> MRRNILLVQFVGVLLLLPSIMSGQQHSSDNKNWAEKGIVIREVEILGKRPMKDIGVQQTRFDSLVLKENIALSMADILTFNSSIFVKSYGRATLSTVSFRGTSASHTQVTWNGMRINNPMLGMTDFSMIPSYFIDDASLLHGTSSVNMAGGGLGGLVKLSTVPAHQEGFGMQYVQGIGSFSTFDEFLQLKYGDKHWQISTRAVYQSSPNDYKYRNHDKKENIYDDKYNIIEQYYPIERNRSGAYKDLHILQEVYYNTGKGDRFGLNAWYTDSNRELALLTTDQGDLMDFENRQREHTLRSVLSWDHTRENWKVSARGGYVHTWLAYDYKRDLGNGIMATMTRSRSKVNTFYGQLDGEYFFSDKLLLTAGVSAHQHLVNSLDKDLNKDDNKNDKYGQGRKNDSIVYFDKGRIELSGNVSLKWQPVNRLGMSLVLRGEMFGTKWAPVIPAFFVDYVLSKRGNIMAKASITRNYRFPTLNDLYFLPGGNPALNNESGFTYETGLSFSVDKDNVYTL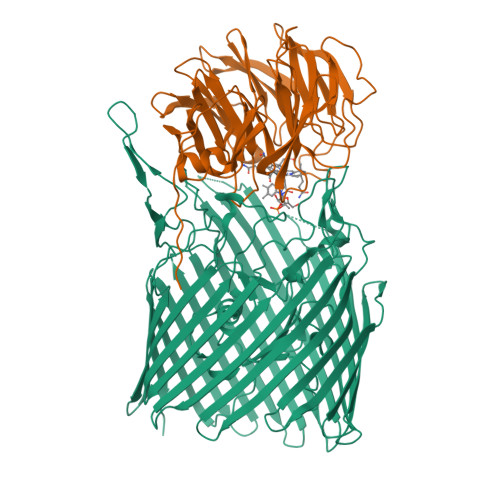SGSASWFDQHINDWIIWLPTSKGFYSPVNLKKVHAYGVEVQADYAVAIDKAWKLGLNGTFAWTPSINEGEPTSKADQSVGKQLPYIPEYSATLSGRLTYRSWGLLYKWCYYSERYTMTSNAVSYTGHLPPYLMSNVTLEKGFSLRWADLSLKGTVNNLFDEEYLSVLSRPMPGINFEFFIGITPKWGKKKKGGGHHHHHH;> MKRILLSVLFIVFCLTAFVGCMKWDYGKMEPFRATGDGLFIMNEGNFQYGNATLSYYDPETKKVENEIFYRANAMKLGDVAQSMIVRDTIGWVVVNNSHVIFAISTNTFKEVGRITGLTSPRYIHFISDEKAYITQIWDYRIFIVNPKTYQITGYIECPDMTMETGSTEQMVQYGKYVYVNCWSYQNRILKIDTTTDKVVDQLTVGIQPTSLVMDKNFKMWTITDGGYKGSPYGYEEPSLYRIDAETFKIEKQFKFQLGDAPSEVQLNGAGDELYWINKDIWRMSVDEERVPVRPFLKYRDTKYYGLTVSPKNGDVYVADAIDYQQQGMIYRYTEDGELVDEFYVGIIPGAFCWK> GSHMPEPTVEDVISQVARAHREIFTYAHDKLGSSPGNFNANHASGSPHGRSGRTVQEIWEDFSMSFTPAVREVVEFAKHIPGFRDLSQHDQVTLLKAGTFEVLMVRFASLFNVKDQTVMFLSRTTYSLQELGAMGMGDLLSAMFDFSEKLNSLALTEEELGLFTAVVLVSADRSGMENSASVEQLQETLLRALRALVLKNRPLETSRFTKLLLKLPDLRTLNNMHSEKLLSFRVDAQ;> THRLITLADHIAQIITQDFA

The nuclear receptor REV-ERB is a component of the molecular clock that regulates the rhythmic expression of inflammatory, metabolic, and cellular proliferative genes. Genes directly regulated by either REV-ERB, REV-ERBα [NR1D1] or REV-ERBβ [NR1D2], are typically transcriptionally silenced by the receptors. This is due to REV-ERB functioning as a ligand-dependent transcriptional repressor with heme as the endogenous ligand. REV-ERBs are particularly efficacious transcriptional repressors, and they lack the carboxy-terminal activation function 2 domain required for coactivator protein recruitment. The REV-ERB LBD displays the canonical NR structure composed of a three-layered α-helical sandwich, and heme binds in the prototypical ligand binding pocket of the LBD.

We determined the crystal structure of a ternary complex containing the REV-ERBα LBD bound to the corepressor NCoR ID1 CoRNR box peptide and the agonist STL1267. Except for helix 12, which is naturally lacking in REV-ERBα, the overall three-dimensional structure of REV-ERBα displays the canonical architecture of nuclear receptor LBD with a three-layer α-helical sandwich and two stranded β-sheets. The C-terminal of helix 11 assumes a well-defined extended β-strand conformation allowing for the formation of an antiparallel β-sheet interactions with N-terminal residues of NCoR ID1. Besides the β-sheet interaction, NCoR ID1 contains a carboxy-terminal four-turn helix that docks into the coregulator binding cleft of REV-ERBα LBD, known as the AF-2 surface. The ligand resides in a predominantly hydrophobic pocket where it makes primarily hydrophobic interactions with the receptor. The triazolo-pyridazine group of STL1267 efficiently fills the narrow portion of the hydrophobic pocket and forms π-π stacking interactions with Phe484 and Phe497. The global receptor conformation of STL1267-bound REV-ERBα LBD was very similar to that of the apo REV-ERBα (overall Cα RMSD of 1.07 Å). First, binding of STL1267 stabilized the β-sheet region (residues Gln493-Gln506) through hydrophobic interactions with Phe497 and Leu498, which is disordered in the apo REV-ERBα structure. The binding of STL1267 is quite distinct from that of heme and where heme binds proximal to helix 11, STL1267 binds distal to helix 11 and is deeply buried within a hydrophobic pocket surrounded by helices 3 and 5 and the two β-sheets strands. STL1267 binding induces an antiparallel β-sheet formation between the amino-terminus of the NCoR ID1 CoRNR box peptide and a β-strand extension of helix 11, which was not observed in the heme-bound receptor.>SSGHMRSTVFSDEEFSNILNDFPALKRNINGKRLVYLDNAASTLKCKSVIEKMTDFYLYHYSNIHRAVHTLASEATVAYEQAREKVANFLNASSEEIIFTSGTTMGINFLVNSLAKSGILKTEDTVLISQVEHHANLVPWVRLSKFYGFKVAYITADEKGVITNESILKTKESIPNPKVVSITGQSNVTGQEMPIELIRETFKNATLIVDGAQLVPHKKVDVKKLDVDFLVFSGHKILGPTGIGVLYGKKALLEQLEPFLYGGEMIDKVTFEDVTFN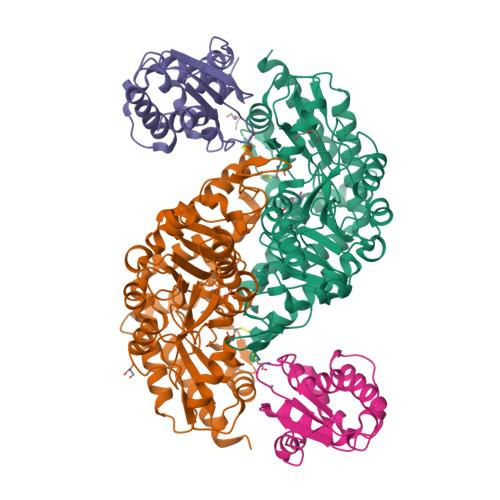VLPYRFEAGTQHITGAVGLGYTIDYLESIGFEKVEKHVEELSNYLLEKMMELDFVEVYGPIDSSHKSLVSFNVKGVHPHDVSHILDENFGVATRSGHHCAQPLMGVLAKGSKIDFPNSTVRASVYLYNTKEDIDVLIEGLKYIRRWFE[2x];>[2x]GSHMIYSEFIMDYSKLKKFHGKIENAHKVEEGKNLSCGDEVTLYFLFDGDKIVDVKFEGHGCAISQASTNVMIEQIIGKTKQEALEMMKNAENMMLGKEFDENVLGPIINFYDVKNYPMRVKCFLLPWKTLEIALKNE> EFPEITEEMEKEIKNVFRNGNQDEVLSEAFRLTITRKDIQTLNHLNWLNDEIINFYMNMLMERSKEKGLPSVHAFNTFFFTKLKTAGYQAVKRWTKKVDVFSV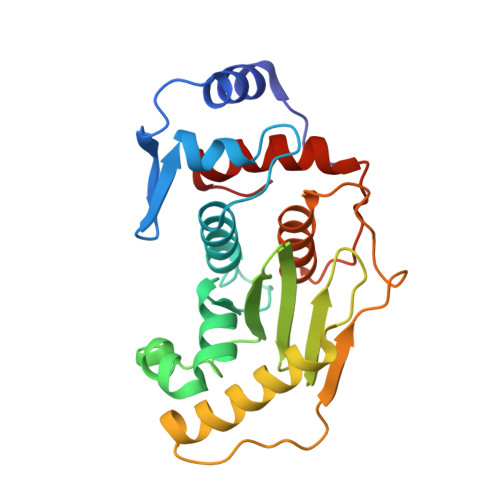DILLVPIHLGVHWCLAVVDFRKKNITYYDSMGGINNEACRILLQYLKQESIDKKRKEFDTNGWQLFSKKSQEIPQQMNGSDCGMFACKYADCITKDRPINFTQQHMPYFRKRMVWEILHRKLL4-[5-[3-[bis(oxidanylidene)-$l^5-sulfanyl]oxyphenyl]-7H-pyrrolo[2,3-d]pyrimidin-4-yl]morpholine 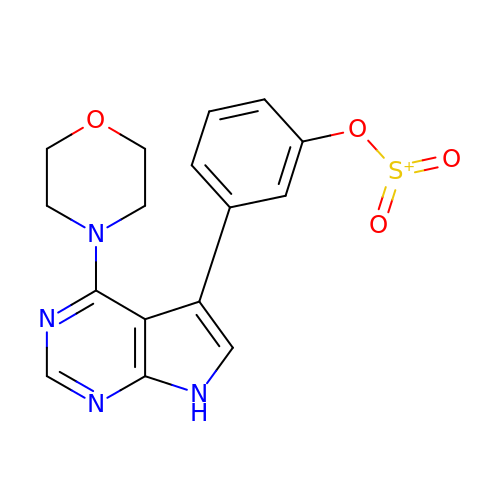| C16 H15 N4 O4 S | WLTPUCQGHKJLHH-UHFFFAOYSA-N In this context, we recently proposed a lanthanide-based molecule, named the crystallophore (Tb-Xo4). Tb-Xo4 is a cationic complex with nucleating and phasing properties. In particular, we show that Tb-Xo4 may provide different crystal forms of a single protein and correct the often-encountered defects in crystalline order that may result in low-resolution data as well as twinning. We prove that, beyond these crystallization properties, Tb-Xo4 is one of the most efficient phasing tools compatible with serial crystallography approaches.

Thia­zole synthase (ThiS) is an enzyme involved in the synthesis of thi­amine diphosphate, a cofactor essential in all life forms for amino acid and carbohydrate metabolism. ThiS consists of a homo-octamer for Methano­coccus jannaschii, and was isolated in fraction C [Fig. 3(a)], where it represents about 40% of the total protein content. Four crystallization conditions corresponding to three different space groups were identified in the absence and presence of Tb-Xo4. Crystal form 1 was obtained in two crystallization conditions. Contrary to FprA which was directly phased from the 10 mM Tb-Xo4 added during crystallization, the co-crystallization of ThiS in the presence of 10 mM Tb-Xo4 was not sufficient to derive useful phases for SAD phasing from crystal form 1. We thus applied a 9 min soaking of one native crystal into a cryo-preserving solution containing 100 mM Tb-Xo4. The model is composed of six protein chains, and 49 Tb sites were modelled with refined occupancies ranging from 0.1 to 0.58. The crystallophore can also be used to directly derive native crystals, as shown for ThiS as well as for the structure determination of vitamin B12 transporter BtuM and the structure of propionyl-CoA synthase from Erythrobacter sp. NAP1.

>[6x]MDYKLKADEYNVTKAILSSAFKMWMDVIEVDVAIVGGGPSGLTAGKYLAKEGLKVVILERHLSFGGGTWGGGMGFPYIVVEEPADEILRDAGIKLEKVEDVEGYYIADSVEVPAKLGASAIDAGAKILTSVAVEDLILREDKVAGVVVQGYAIEKAGLHVDPITINAKYVIDATGHDASVTTTLARKNKDLGIEVPGEKSMWADKGENSLLRNTREVYPGLFVCGMAANAVHAGYRMGAIFGGMYLSGKKCAEMILEKLNK The IRG1 protein, also known as CAD, is over-expressed during immune responses and catalyzes the production of itaconate, which functions as an immunometabolite possessing antibacterial, antiviral, and immunoregulatory activities. In mammalian systems, itaconate production is catalyzed by immune responsive gene 1 (IRG1), which is known as an LPS-inducible protein highly expressed during the inflammation phase of pathogen infection. Itaconate, the decarboxylated product of cis-aconitate (an intermediate metabolite in the TCA cycle), is a small immunometabolite that can control innate immunity and possesses antibacterial and antiviral activity. Our findings indicate that IRG1 exist as a dimer in solution.

The detected asymmetric unit contained two molecules (A and B), which comprise the functional unit of IRG1. Following the refinement and model building process, the model of molecule A was constructed from residues 5 to 463 and the model of molecule B was constructed from residues 4 to 460. The mouse IRG1 structure revealed that it is composed of two distinct domains, a helical domain and lid domain. The helical domain is formed by 270 N-terminal and 80 C-terminal residues, while the lid domain is formed by 140 residues in the middle of mouse IRG1. Interestingly, an unknown electron density was observed in the active site of our IRG1 structure. All the side chains of the amino acid residues forming the active site were orientated towards the unidentified density. Based on this observation, we hypothesized that unknown density (might be from substrate: this also suggested by Chen et al) fixed the close conformation of IRG1 by holding the A1 loop. Structural analysis in this area showed that K152 and D153 from A1 loop formed hydrogen bonds with S381 from A2 loop.

>MMLKSVTESFAGMIHGLKVNHLTDGIIRRSKRMILDSLGVGFLGTGTEVFHKVTQYSKIYSSNTSSTVWGRPDFRLPPTYAAFVNGVAVHSMDFDDTWHPATHPSGAVLPVLTALSEALPQTPKFSGLDLLLAFNVGIEVQGRLMHFSKEAKDIPKRFHPPSVVGTLGSAAAASKFLGLSLTKCREALAIAVSHAGAPIANAATQTKPLHIGNAAKHGMEATFLAMLGLQGNKQILDLGSGFGAFYANYSPEDLPSLDSHIWLLDQQDVAFKSFPAHLATHWVADAAAAVRKHLVTPERALFPADHIERIVLRIPDVQYVNRPFPDSEHEARHSFQYVACASLLDGSITVPSFHSQQVNRPQVRELLKKVKLEHPPDNPPSFDTLYCEISITLKDGTTFTERSDTFYGHWRKPLSQEDLRNKFRANASKMLCRDTVESLITVVEKLEDLEDCSVLTRLLKGPSVQDEASKLSSMSSFDHTTLPRFTNI[2x]>[2x]MKTSTTYGGESLTEAYLYYFNQICEDAREAAYSYYFDGSGNFKSTYIGGKVSPQNEPKRIWDDLTAGHITQDEAKDRILSGMREIIVSEVNNFMNGLPSSISFKVSPSSPITINKLDDLKNYILKELKDISNFGVGSFTVSSWSAGDVKGYTVEFEVYKEQNTGTSPAKDTVRNMRIDIAVNKGVMPDIGTLNPTSSTSSWNDLFEYAVYSRGSFLPNYKFTVRGGSIYSGERIQTQGEFKAIGVNNLICKGPEVIVNGGGNSIEIKEIMYIQNKLVFNGAPNTNPNTLNANKIY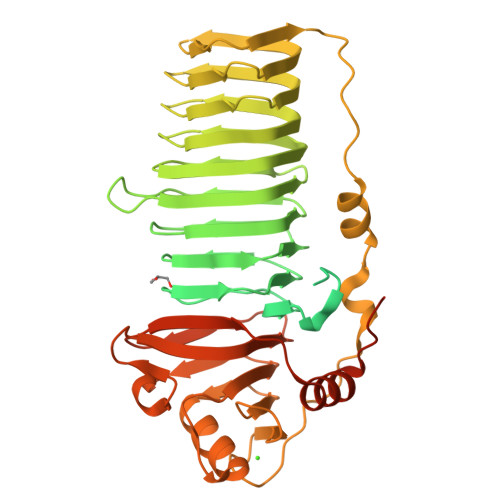TGLGGMELNGYGYYKANEIYSDGEVQVKNYGNFEIGSIGIVKKLTVTDNGRTTIKSGATLYCDQLEVRNNGRVFIEAGATLVTRAISISGGTIEGPGTRQVNPSATFPSYPPFIDDIKNFDFDSRMSVTTLPADPVGATTLGSVYDKSATPWEIVVYGESGINDSELITEVNSKLGSFPSNVRLYLASKGNITFSNPTSLPLYNPTTGKLVIEGAIITLGSTFNINISGAGIELIYKRAGSTIESSITSTLNYIPPPRSYSSSSAQTVNTMYQVKRRGMIIK>UCGUACGA[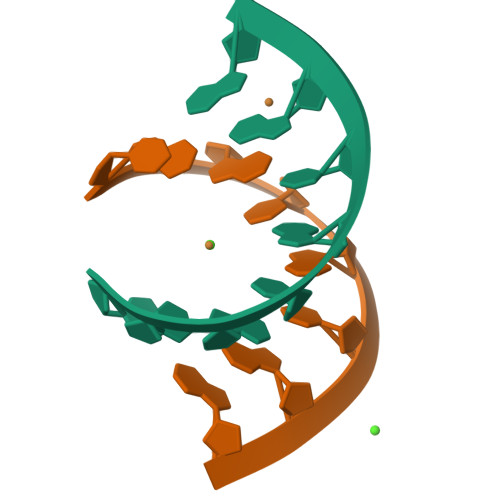2x]> KDGDQCETSP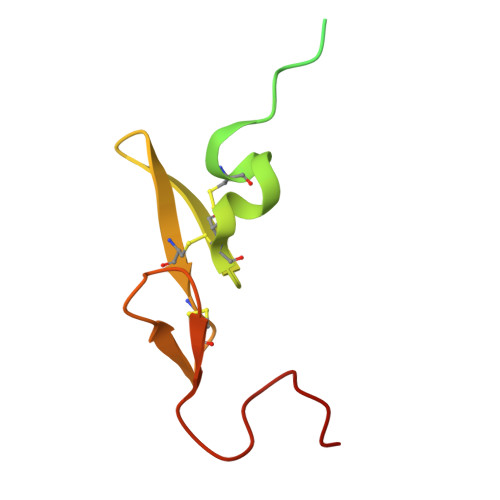CQNQGKCKDGLGEYTCTCLEGFEGKNCELFTRKLCSLDNGDCDQFCHEEQNSVVCSCARGYTLADNGKACIPTGPYPCGKQTLE>[2x]MVKE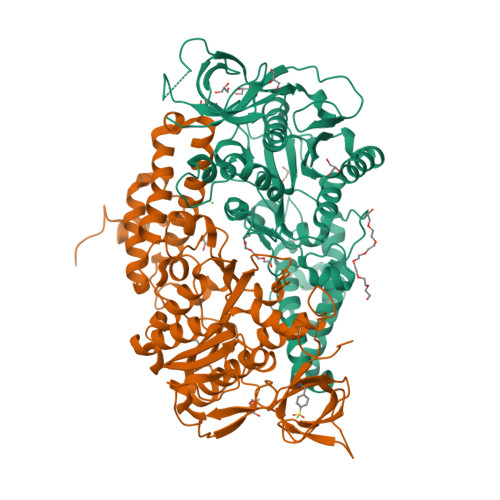YKTITQIAGPLIFVEKTEPVGYNEIVNIKMGDGTVRRGQVLDSSADIVVVQVFEGTGGLDKDCGVIFTGETLKLPASVDLLGRILSGSGEPRDGGPRIVPDQLLDINGAAMNPYARLPPKDFIQTGISTIDGTNTLVRGQKLPIFSASGLPANEIALQIARQASVPGSESAFAVVFAAMGITNEEAQYFMSDFEKTGALERAVVFLNLADDPAVERIVTPRMALTAAEYLAYEHGMHVLVILTDITNYAEALRQMGAARNEVPGRRGYPGYMYTDLATLYERAGIVKGAKGSVTQIPILSMPGDDITHPIPDLSGYITEGQIVVARELHRKGIYPPINVLPSLSRLMNSGIGAGKTREDHKAVSDQMYAGYAEGRDLRGLVAIVGKEALSERDTKFLEFADLFEDKFVRQGRNENRTIEDTLEIGWQILTHLPENQLGRIDNKYIQKYHPAHRKAK(2S,3S)-3-{3-[4-(METHYLSULFONYL)PHENYL]-1,2,4-OXADIAZOL-5-YL}-1-OXO-1-PYRROLIDIN-1-YLBUTAN-2-AMINE 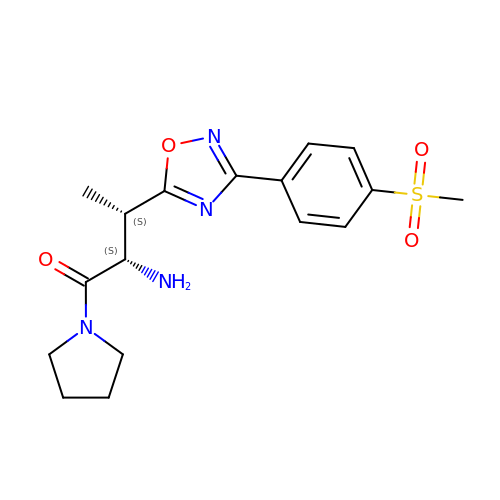| C17 H22 N4 O4 S | SQCDMTZMCHZYGO-FZMZJTMJSA-N>[4x]MEGPAGYLRRASVAQLTQELGTAFFQQQQLPAAMADTFLEHLCLLDIDSEPVAARSTSIIATIGPASRSVERLKEMIKAGMNIARLNFSHGSHEYHAESIANVREAVESFAGSPLSYRPVAIALDTKGPEIRTGILQGGPESEVELVKGSQVLVTVDPAFRTRGNANTVWVDYPNIVRVVPVGGRIYIDDGLISLVVQKIGPEGLVTQVENGGVLGSRKGVNLPGAQVDLPGLSEQDVRDLRFGVEHGVDIVFASFVRKASDVAAVRAALGPEGHGIKIISKIENHEGVKRFDEILEVSDGIMVARGDLGIEIPAEKVFLAQKMMIGRCNLAGKPVVCATQMLESMITKPRPTRAETSDVANAVLDGADCIMLSGETAKGNFPVEAVKMQHA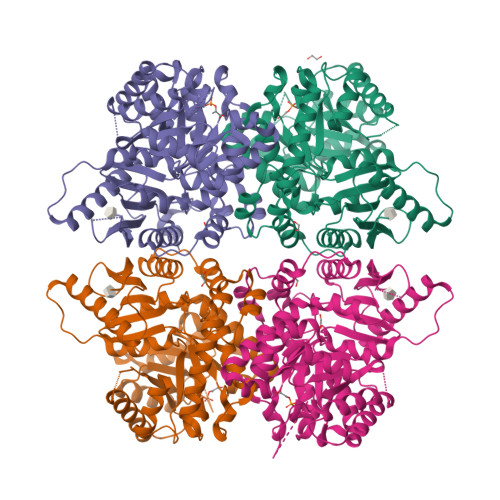IAREAEAAVYHRQLFEELRRAAPLSRDPTEVTAIGAVEAAFKCCAAAIIVLTTTGRSAQLLSRYRPRAAVIAVTRSAQAARQVHLCRGVFPLLYREPPEAIWADDVNRRVQFGIESGKLRGFLRVGDLVIVVTGWRPGSGYTNIMRVLSIS Recently, we characterized TgCyp23 among the various Cyps of the parasite, demonstrating its high PPIase activity and its ability to bind cyclosporin A (CsA), a well‐known inhibitor of Cyps (Favretto et al., 2023). TgCyp23 exhibits the typical eight‐stranded antiparallel β‐barrel structure, with two α‐helices flanking the barrel on either side, all of them connected by loops. TgCyp23 shows remarkable sequence identity with human CypA (~52% of identity) but has a 40‐aminoacid N‐terminal extension. Here, three new structures of the protein in complex with the three non‐immunosuppressive derivatives NIM811, dhCsA, and Alisporivir have been solved at 1.17, 1.20, and 1.20 Å resolution, respectively.

Alisporivir (Debio 025) differs from CsA in the residues at positions 3 and 4. It replaces the sarcosine (Sar‐3) moiety at position 3 and MeLeu‐4 residue at position 4 with N‐methyl‐D‐Alanine (MeAla‐3) and N‐ethylvaline (NEV‐4), respectively. Thr117 exhibits a displacement of 1 Å in the carbon backbone, a phenomenon anticipated due to Alisporivir's additional methyl group at position 3. This alteration induces a slight shift in the L108–140 loop, with the most notable effect observed in the residue Thr117, the nearest amino acid to the methyl group. Specifically, Alisporivir displayed the highest interaction affinity with TgCyp23 (Kd = 15 ± 3 nM) while dhCsA showed the lowest affinity (Kd = 200 ± 92 nM). Of note, the affinity of Alisporivir surpassed that of CsA (Kd = 82 ± 15 nM) (Favretto et al., 2023). Comparison of the CsA and Alisporivir complexes structures allowed us to rationalize the higher affinity of Alisporivir, revealing subtle effects due to the introduction of N‐methyl group at position 3. This modification induces the formation of superior Van der Waals contacts between the unique side chain of the ligand and TgCyp23 (T117 residue) and causes protein structural rearrangements, specifically within loops L108–140 and L144–156. Similarly to NIM811, in Alisporivir, the side chain of NEV‐4 creates steric hindrance, preventing it from occupying the hydrophobic Cn cavity and proper interactions.

>[2x]GHMAPAPPANSGESSLLSESELPAGISYAEAMEGGSRPLLHPDNPVVFFDISIGSHEAGRIKIELFKNLAPKSAENFRQFCTGEFRQNQVPIGYKGATFHRIIKNFMIQGGDFVKGDGTGRLSIYGSSFPDEAFVLPHFRSGLLSLANSGPDTNGCQFFITCAKCDWLNRKHVVFGQVLGKESMQVVRKIEHVTVDGGNRPRIPVTVTQCGEL;>ALLVTAAXVLA[2x]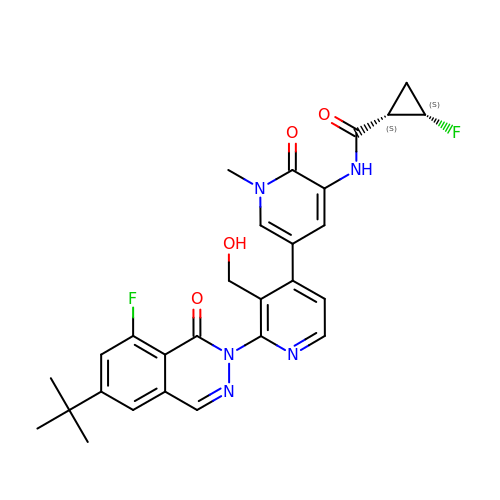(1S,2S)-N-[2'-(6-tert-butyl-8-fluoro-1-oxophthalazin-2(1H)-yl)-3'-(hydroxymethyl)-1-methyl-6-oxo[1,6-dihydro[3,4'-bipyridine]]-5-yl]-2-fluorocyclopropane-1-carboxamide | C28 H27 F2 N5 O4 | SEGFWFQHVPYNMS-QUCCMNQESA-N>[2x]MTLGDLWKRKLNGCTKEEFFAYRRTGILETERDKARELLRRGETNMGLAVSRGTAKLAWLEERGYATLKGEVVDLGCGRGGWSYYAASRPAVMSVKAYTIGGKGHETPKMVTSLGWNLIKFRAGMDVFSMQPHRA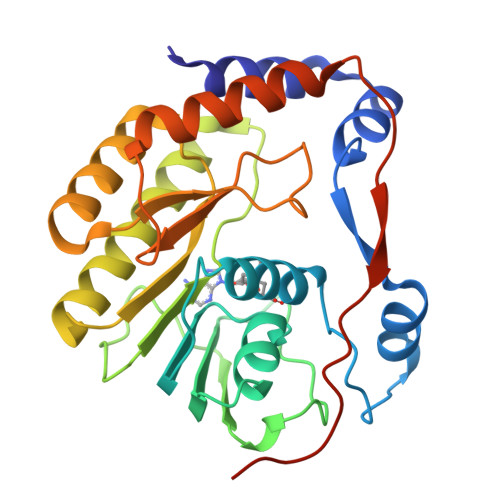DTIMCDIGESNPDAVVEGERTRKVILLMEQWKNRNPTATCVFKVLAPYRPEVIEALHRFQLQWGGGLVRTPFSRNSTHEMYYSTAVTGNIVNSVNIQSRKLLARFGDQRGPTRVPELDLGVGTRGSSSHHHHHH> PIETVPVKLKPGMDGPKVKQWPLTEEKIKALVEICTEMEKEGKISKIGPENPYNTPVFAIKKKDSTKWRKLVDFRELNKRTQDFWEVQLGIPHPAGIKKKKSVTVLDVGDAYFSVPLDEDFRKYTAFTIPSINNETPGIRYQYNVLPQGWKGSPAIFQSSMTKILEPFRKQNPDIVIYQYMDDLYVGSDLEIGQHRTKIEELRQHLLRWGLTTPDKKHQK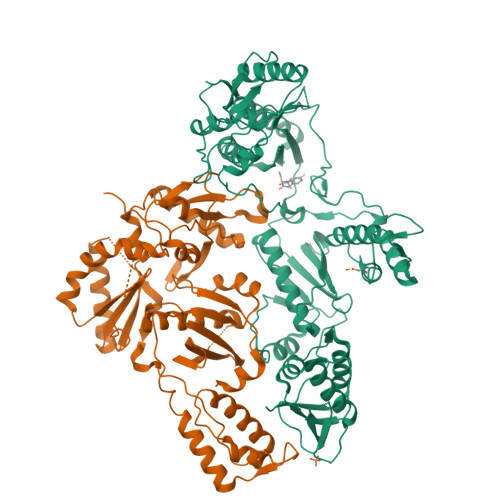EPPFLWMGYELHPDKWTVQPIVLPEKDSWTVNDIQKLVGKLNWASQIYPGIKVRQLCKLLRGTKALTEVIPLTEEAELELAENREILKEPVHGVYYDPSKDLIAEIQKQGQGQWTYQIYQEPFKNLKTGKYARMRGAHTNDVKQLTEAVQKITTESIVIWGKTPKFKLPIQKETWETWWTEYWQATWIPEWEFVNTPPLVKLWYQLEKEPIVGAETFYVDGAANRETKLGKAGYVTNRGRQKVVTLTDTTNQKTELQAIYLALQDSGLEVNIVTDSQYALGIIQAQPDQSESELVNQIIEQLIKKEKVYLAWVP;> IETVPVKLKPGMDGPKVKQWPLTEEKIKALVEICTEMEKEGKISKIGPENPYNTPVFAIKKKDSTKWRKLVDFRELNKRTQDFWEVQLGIPHPAGIKKKKSVTVLDVGDAYFSVPLDEDFRKYTAFTIPSINNETPGIRYQYNVLPQGWKGSPAIFQSSMTKILEPFRKQNPDIVIYQYMDDLYVGSDLEIGQHRTKIEELRQHLLRWGLTTPDKKHQKEPPFLWMGYELHPDKWTVQPIVLPEKDSWTVNDIQKLVGKLNWASQIYPGIKVRQLCKLLRGTKALTEVIPLTEEAELELAENREILKEPVHGVYYDPSKDLIAEIQKQGQGQWTYQIYQEPFKNLKTGKYARMRGAHTNDVKQLTEAVQKITTESIVIWGKTPKFKLPIQKETWETWWTEYWQATWIPEWEFVNTPPLVKLWYQ>MTGMSREEVESLIQEVLEVYPEKARKDRNKHLAVNDPAVTQSKKCIISNKKSQPGLMTIRGCAYAGSKGVVWGPIKDMIHISHGPVGCGQYSRAGRRNYYIGTTGVNAFVTMNFTSDFQEKDIVFGGDKKLAKLIDEVETLFPLNKGISVQSECPIGLIGDDIESVSKVKGAELSKTIVPVRCEGFRGVSQSLGHHIANDAVRDWVLGKRDEDTTFASTPYDVAIIGDYNIGGDAWSSRILLEEMGLRCVAQWSGDGSISEIELTPKVKLNLVHCYRSMNYISRHMEEKYGIPWMEYNFFGPTKTIESLRAIAAKFDESIQKKCEEVIAKYKPEWEAVVAKYRPRLEGKRVMLYIGGLRPRHVIGAYEDLGMEVVGTGYEFAHNDDYDRTMKEMGDSTLLYDD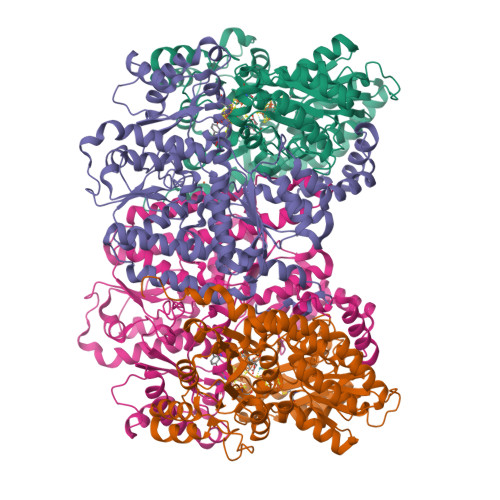VTGYEFEEFVKRIKPDLIGSGIKEKFIFQKMGIPFREMHSWDYSGPYHGFDGFAIFARDMDMTLNNPCWKKLQAPWEASEGAEKVAASA[2x];>[2x]MSQQVDKIKASYPLFLDQDYKDMLAKKRDGFEEKYPQDKIDEVFQWTTTKEYQELNFQREALTVNPAKACQPLGAVLCALGFEKTMPYVHGSQGCVAYYRSYFNRHFREPVSCVSDSMTEDAAVFGGQQNMKDGLQNCKATYKPDMIAVSTTCMAEVIGDDLNAFINNSKKEGFIPDEFPVPFAHTPAFVGSHVTGWDNMFEGIARYFTLKSMDDKVVGSNKKINIVPGFETYLGNFRVIKRMLSEMGVGYSLLSDPEEVLDTPADGQFRMYAGGTTQEEMKDAPNALNTVLLQPWHLEKTKKFVEGTWKHEVPKLNIPMGLDWTDEFLMKVSEISGQPIPASLTKERGRLVDMMTDSHTWLHGKRFALWGDPDFVMGLVKFLLELGCEPVHILCHNGNKRWKKAVDAILAASPYGKNATVYIGKDLWHLRSLVFTDKPDFMIGNSYGKFIQRDTLHKGKEFEVPLIRIGFPIFDRHHLHRSTTLGYEGAMQILTTLVNSILERLDEETRGMQATDYNHDLVR>GPMSEAADVERVYAAMEEAAGLLGVACARDKIYPLLSTFQDTLVEGGSVVVFSMASGRHSTELDFSISVPTSHGDPYATVVEKGLFPATGHPVDDLLA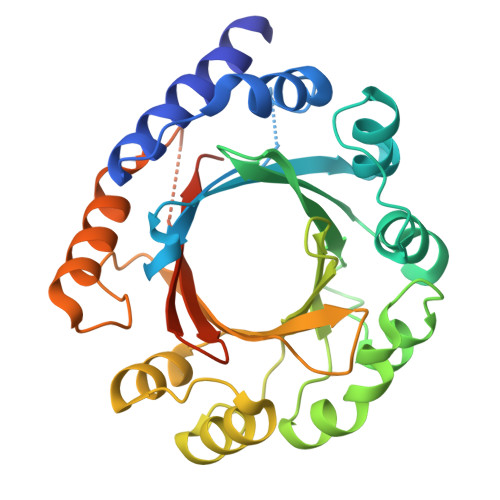DTQKHLPVSMFAIDGEVTGGFKKTYAFFPTDNMPGVAELSAIPSMPPAVAENAELFARYGLDKVQMTSMDYKKRQVNLYFSELSAQTLEAESVLALVRELGLHVPNELGLKFCKRSFSVYPTLNWETGKIDRLCFAVISNDPTLVPSSDEGDIEKFHNYATKAPYAYVGEKRTLVYGLTLSPKEEYYKLGAPYHITDVQRGLLKAFDSLED[4x]> GAMGALPPDGHPVEPH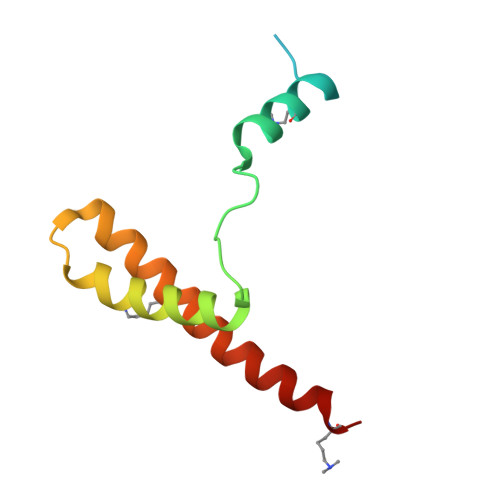LERLYPTAQSKRSLWDFASPGYTFHGLHRAQDYRRELDTLQSLLTTSQSSELQAAAALLKCQQDDDRLLQIILNLLHKV>GAMPHDPSFTPTQLAARAAYLLRGNDLGTMTTAAPLLYPHMWSWDAAFVAIGLAPLSVERAVVELDTLLSAQWRNGMIPHIVFANGVDGYFPGPARWATATLADNAPRNRLTSGITQPPVHAIAVQRILEHARTRGRSTRAVAEAFLDRRWGDLMRWHRWLAECRDRNERGRITLYHGWESGMANSPRWDSAYANVVPGKLPEYQRADNVIITDPSQRPSDGEYDRYLWLLEEMKAVRYDDERLPSVMSFQVEDVFFSAIFSVACQVLAEIGEDYKRPHADVKDLYLWAERF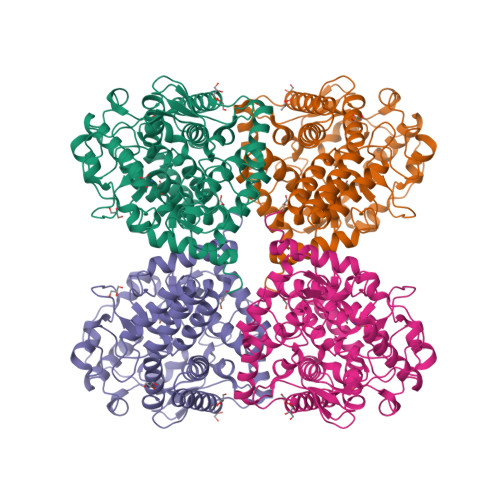RAGVVETTDQRTGAARDFDVLAEKWLVTETAAQFAPLLCGGLPHDRERALLKLLEGPRFCGHPDLKYGLIPSTSPVSRDFRPREYWRGPVWPVLTWLFSWCFARRGWAERARLLRQEGLRQASDGSFAEYYEPFTGEPLGSMQQSWTAAAVLDWLG[2x]>TRDQNGTWEMESNENFEGYMKALDIDFATRKIAVRLTQTKVIDQDGDNFKTKTTSTFRNWDVDFTVGVEFDEYTKSLDNRHVKALVTWEGDVLVCVQKGEKENRGWKQWIEGDKLYLELTCGDQVCRQVFKKK[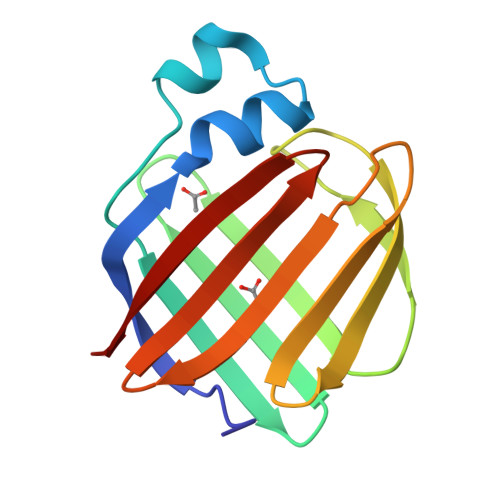4x]>[2x]SASIEKVNKLPKSPRNRFLLPPKGGTETTRRDIYNQILKDMAAFPENTIVTAVLASVDVTDNCAYVAKWDESSDRIKKVLQRQLPLQELDQLPDYGDIFAVLDSINNIITRITIN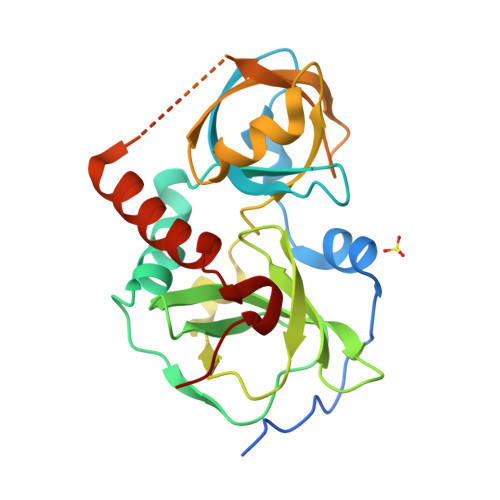SSSAGGGYDAYLIDFGEHIHFDGNETIFKLPDDIKRLPAQAIRCDLINCDIANMHCFVNTYIKIRVHENNNSTLVAEPVIDRLSRPTKTNTTKYPAGITEDDMAMLNEIDESTSDPLKAVLGFRPKD>AGKKVLIVYAHQEPKSFNGSLKNVAVDELSRQGCTVTVSDLYAMNFEPRATDKDITGTLSNPEVFNYGVETHEAYKQRSLASDITDEQKKVREADLVIFQFPLYWFSVPAILKGWMDRVLCQGFAFDIPGFYDSGLLQGKLALLSVTTGGTAEMYTKTGVNGDSRYFLWPLQHGTLHFCGFKVLAPQISFAPEIASEEERKGMVAAWSQRL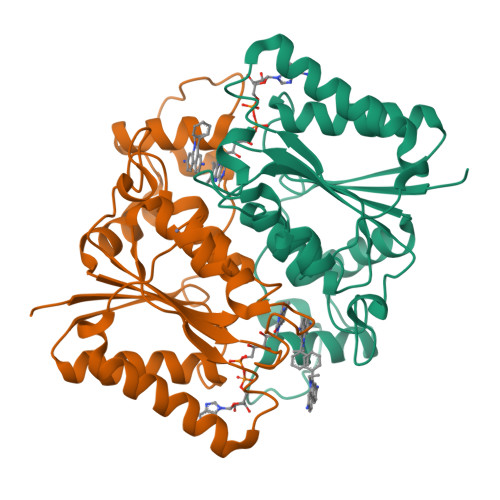QTIWKEEPIPCTAHWHFGQ[2x]> SNAMNKVITDLDKALSALKDGDTILVGGFGLCGIPEYAIDYIYKKGIKDLIVVSNNCGVDDFGLGILLEKKQIKKIIASYVGENKIFESQMLNG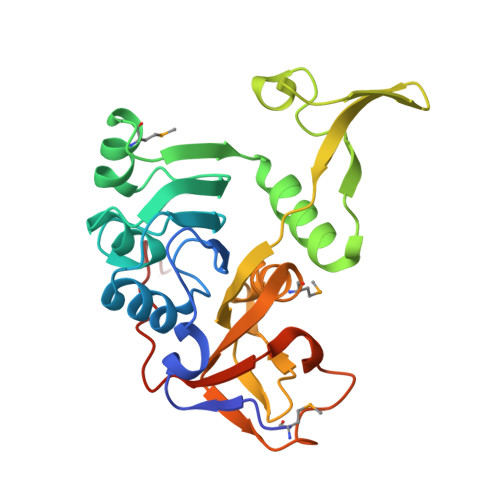EIEVVLTPQGTLAENLHAGGAGIPAYYTPTGVGTLIAQGKESREFNGKEYILERAITGDYGLIKAYKSDTLGNLVFRKTARNFNPLCAMAAKICVAEVEEIVPAGELDPDEIHLPGIYVQHIYKGEKFEKRIEKITTRSTK>[2x]MPRQASTFTNPVLWEDHPDLEVFRVGSVFYYSSSTFAYSPGAPVLKSYDLVHWTPVTHSVPRLNFGSNYDLPSGTPGAYVKGIWASTLRYRRSNDRFYWYGCVEGRTYLWTSPGGNALANNGEVPPSAWNWQHTATIDNCYADAGLLIDDDDTMYIAYGNPTIN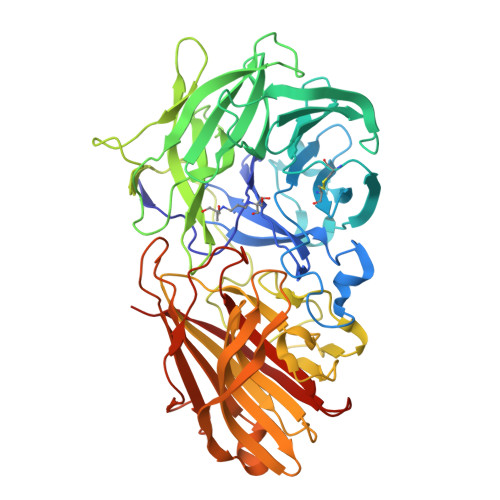VAQLSPDGTRQVRVQQRVYAHPQGQTVAGARMYKIRGNYYILVTRPADAEYVLRSTTGSPFGPYEARTLVSRIQGPLANAGFAHQGGIVDAPDGTWHYVAFMDAYPGGRIPVVAPLRWTADGWPEVVTDSQGRWGTSYPIPVRGAKNATEGLASTDLDEFRGTRFSEHWEWNHNPDTSKFTLLGGNEGGLILRTATVTGDLFAARNTLTRRIAGPKASGIFRLDVRGMRDGDRAGAVLFRDRAAYIGVWKQGNEARIVMVDDLRLNEDGWRTASTGRVAANGPVIDTNAQQDIWLRIDADITPAFGTNTERTTTFYYSIDGGRTYTRLGPAFAMTNSWRYFTGYRFGVFNFSTKSLGGEVKVKGFKMNMILEHHHHHH> MTGGMKPPARKPRILNSDGSSNITRLGLEKRGWLDDHYHDLLTVSWPVFITLITGLYLVTNALFALAYLACGDVIENARPGSFTDAFFFSVQTMATIGYGKLIPIGPLANTLVTLEALCGMLGLAVAASLIYARFTRPTAGVLFSSRMVISDFEGKPTLMMRLANLRIEQIIEADVHLVLVRSEISQEGMVFRRFHDLTRTRSRSPIFSLSWTVMHPIDHHSPIYGETDETLRNSHSEFLVLFTGHHEAFAQNVHARHAYSCDEIIWGGHFVDVFTTLPDGRRALDLGKFHEIAQHHHHHH;> MTGGMKPPARKPRILNSDGSSNITRLGLEKRGWLDDHYHDLLTVSWPVFITLITGLYLVTNALFALAYLACGDVIENARPGSFTDAFFFSVQTMATIGYGKLIPIGPLANTLVTLEALCGMLGLAVAASLIYARFTRPTAGVLFSSRMVISDFEGKPTLMMRLANLRIEQIIEADVHLVLVRSEISQEGMVFRRFHDLTLTRSRSPIFSLSWTVMHPIDHHSPIYGETDETLRNSHSEFLVLFTGHHEAFAQ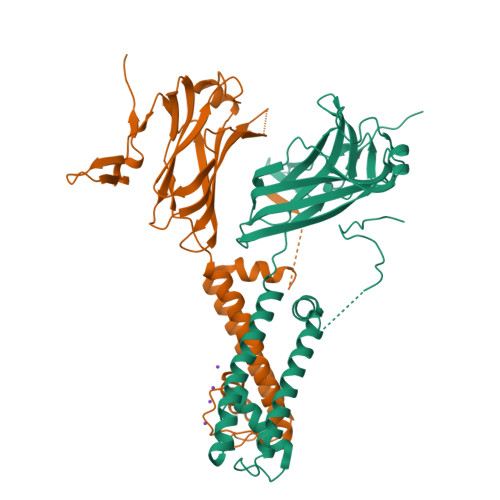NVHARHAYSCDEIIWGGHFVDVFTTLPDGRRALDLGKFHEIAQHHHHHH>[2x]MDYEKFLLFGDSITEFAFNTRPIEDGKDQYALGAALVNEYT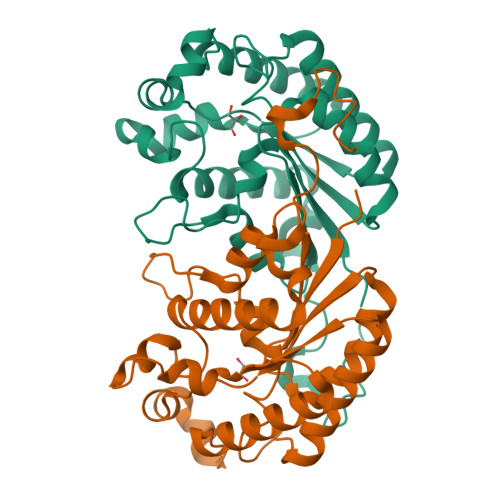RKMDILQRGFKGYTSRWALKILPEILKHESNIVMATIFLGANDACSAGPQSVPLPEFIDNIRQMVSLMKSYHIRPIIIGPGLVDREKWEKEKSEEIALGYFRTNENFAIYSDALAKLANEEKVPFVALNKAFQQEGGDAWQQLLTDGLHFSGKGYKIFHDELLKVIETFYPQYHPKNMQYKLKDWRDVLDDGSNIMSLE> GPMEQLKHCNGILKELLSKKHAAYAWPFYKPVDASALGLHDYHDIIKHPM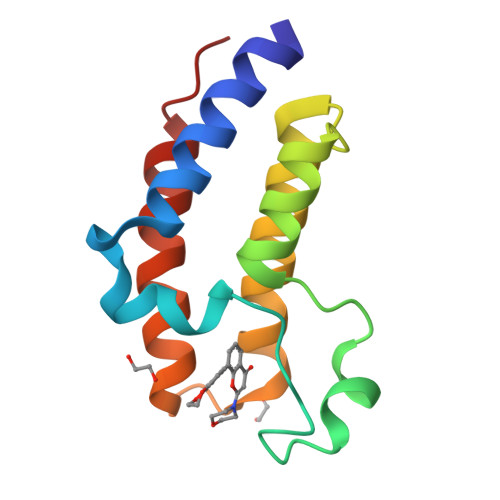DLSTVKRKMENRDYRDAQEFAADVRLMFSNCYKYNPPDHDVVAMARKLQDVFEFRYAKMPD4-[3-(2-amino-4-hydroxy-6-oxo-1,6-dihydropyrimidin-5-yl)propyl]benzoic 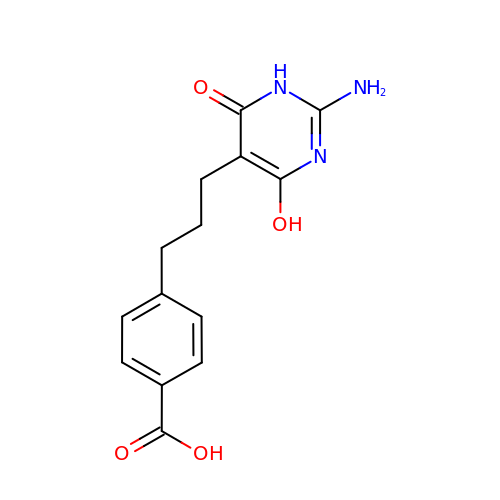acid | C14 H15 N3 O4 | GBBVOAWLGQEGEW-UHFFFAOYSA-N> AEFGSHHHHHHGSAPMAEGGGQNHHEVVKFMDVYQRSYCHPIETLVDIFQEYPDEIEYIFKPSCVPLMRCGGCCNDEGLECVPTEESNITMQIMRIKPHQGQHIGEMSFLQHNKCECRPKKDRARQENCDKPRR;> MQSKVLLAVALWLCVETRAASVGLPSVSLDLPRLSIQKDILTIKANTTLQITCRGQRDLDWLWPNNQSGSEQRVEVTECSDGLFCKTLTIPKVIGNDTGAYKCFYRETDLASVIYVYVQDYRSPFIASVSDQHGVVYITENKNKTVVIPCLGSISNLNVSLCARYPEKRFVPDGNRISWDSKKGFTIPSYMISYAGMVFCEAKINDESYQSIMYIVVVVGYRIYDVVLSPSHGIELSVGEKLVLNCTARTELNVGIDFNWEYPSSKHQHKKLVNRDLKTQSGSEMKKFLSTLTIDGVTRSDQGLYTCAASSGLMTKKNSTFVRVHEKPFVAFGSGMESLVEATVGERVRIPAKYLGYPPPEIKWYKNGIPLESNHTIKAGHVLTIMEVSERDTGNYTVILTNPISKEKQSHVVSLVVYVPPQIGEKSLISPVDSYQYGTTQTLTCTVYAIPPPHHIHWYWQLEEECANEPSQAVSVTNPYPCEEWRSVEDFQGGNKIEVNKNQFALIEGKNKTVSTLVIQAANVSALYKCEAVNKVGRGERVISFHVTRGPEITLQPDMQPTEQESVSLWCTADRSTFENLTWYKLGPQPLPIHVGELPTPVCKNLDTLWKLNATMFSNSTNDILIMELKNASLQDQGDYVCLAQDRKTKKRHCVVRQLTVLERVAPTITGNLENQT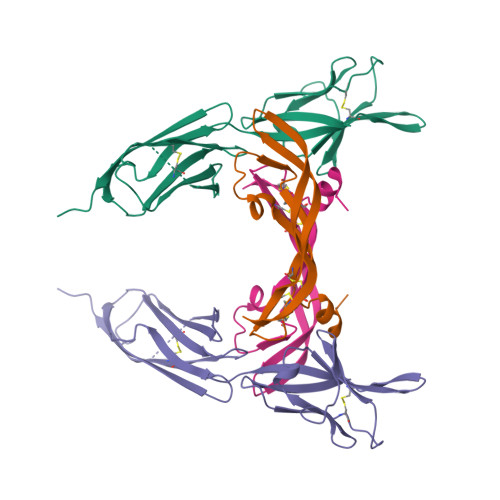TSIGESIEVSCTASGNPPPQIMWFKDNETLVEDSGIVLKDGNRNLTIRRVRKEDEGLYTCQACSVLGCAKVEAFFIIEGAQEKTNLERTHHHHHH(3S)-3-[(3R)-1-acetylpiperidin-3-yl]-6-chloro-3-(3-chlorobenzyl)-1,3-dihydro-2H-indol-2-one 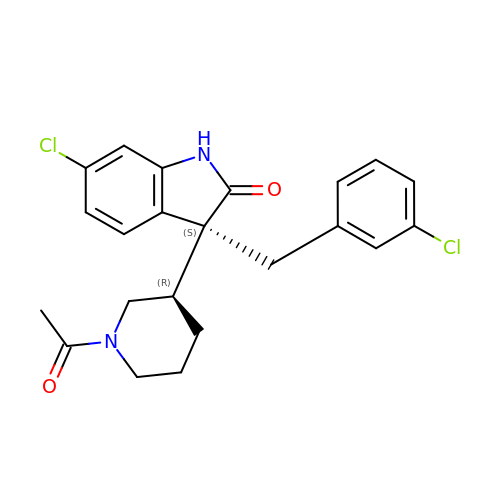| C22 H22 Cl2 N2 O2 | RIBYLXUNNWIWJK-AOMKIAJQSA-N>[2x]GPGSMIKIHTEKDFIKMRAAGKLAAETLDFITDHVKPNVTTNSLNDLCHNFITSHNAIPAPLNYKGFPKSICTSINHVVCHGIPNDKPLKNGDIVNIDVTVILDGWYGDTSRMYYVGDVAIKPKRLIQVTYDAMMKGIEVVRPGAKLGDIGYAIQSYAE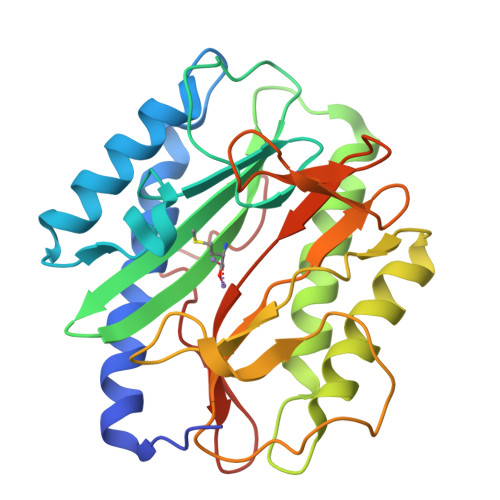KHNYSVVRDYTGHGIGRVFHDKPSILNYGRNGTGLTLKEGMFFTVEPMINAGNYDTILSKLDGWTVTTRDKSLSAQFEHTIGVTKDGFEIFTLSPKKLDYPPY N-[(1S)-1-benzyl-2-(3-guanidinopropylamino)-2-oxo-ethyl]-4-hydroxy-2-oxo-1H-quinoline-6-carboxamide | C23 H26 N6 O4 | 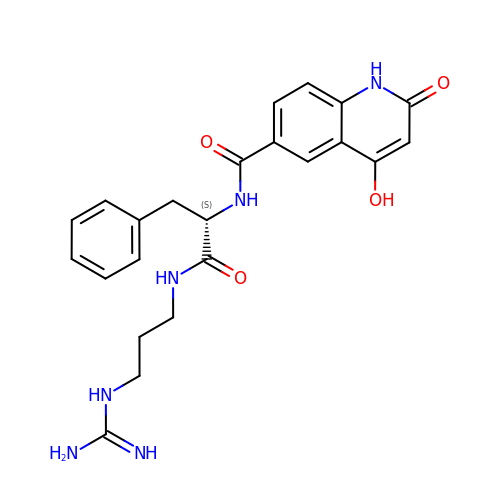JBDCCMFGOOWYSC-SFHVURJKSA-N> MSRSKRDNNFYSVEIGDSTFTVLKRYQNLKPIGSGAQGIVCAAYDAILERNVAIKKLSRPFQNQTHAKRAYRELVLMKCVNHKNIIGLLNVFTPQKSLEEFQDVYIVME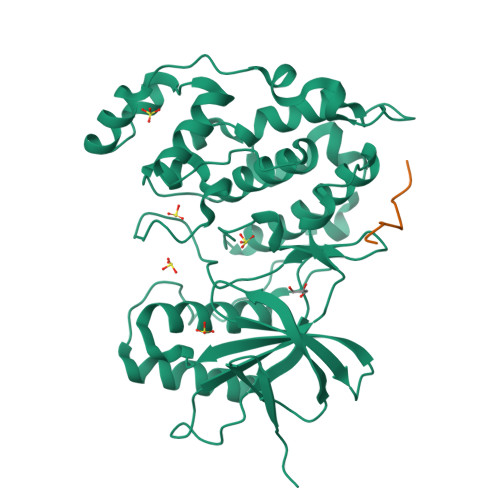LMDANLSQVIQMELDHERMSYLLYQMLCGIKHLHSAGIIHRDLKPSNIVVKSDATLKILDFGLARTAGTSFMMTPYVVTRYYRAPEVILGMGYKENVDIWSVGCIMGEMIKGGVLFPGTDHIDQWNKVIEQLGTPSPEFMKKLQPTVRTYVENRPKYAGYSFEKLFPDVLFPADSEHNKLKASQARDLLSKMLVIDASKRISVDEALQHPYINVWYDPSEAEAPPPKIPDKQLDEREHTIEEWKELIYKEVMDLEHHHHHH;> RPKRPTTLNLF>ADATDDYPIPNRIMRTPCTAEQIMAAARDVEPVYYERYMTDYKNKPPHVQQAARDRIHWFFSMDYAGRRQYSENTATDAFFEQLAWMWPNWAKLFFNNKGVAANTTDVCEQYPPDDMS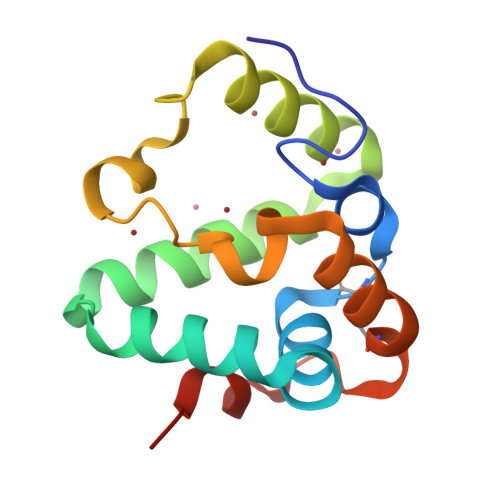VWNWDDDDK[2x]methyl 2-methylprop-2-enoate | C5 H8 O2 | 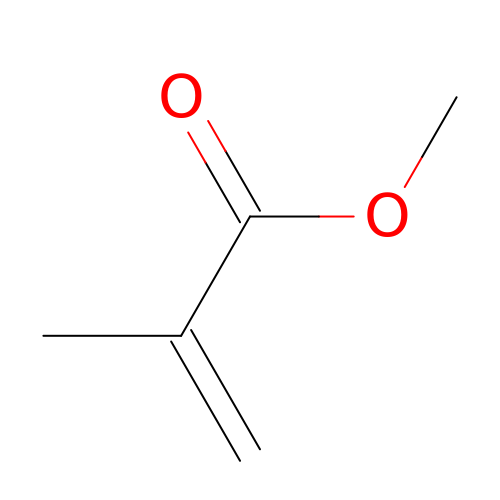VVQNEPGJFQJSBK-UHFFFAOYSA-N> SMDESGLPQLTSYDCEVNAPIQGSRNLLQGEELLRALDQ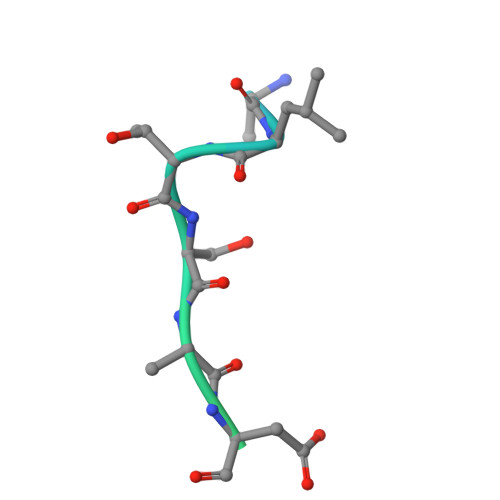VN>[2x]GGGAEALELLEHCGVCRERLRPEREPRLLPCLHSACSACLGPAAPAAANSSGDGGAAGDGTVVDCPVCKQQCFSKDIVENYFMRDSGSKAATDAQDANQCCTSCEDNAPATSYCVECSEPLCETCVEAHQRVKYTKDHTVRSTGPAKSRDGERTVYCNVHKHEPLVLFCESCDTLTCRDCQLNAHKDHQYQFLEDAVRNQRKLLASLVKRLGDKHATLQKSTKEVRSSIRQVSDVQKRVQVDVKMAILQIMKELNKRGRVLVNDAQKVTEGQQERLERQHWTMTKIQKHQEHILRFASWALESDNNTALLLSKKLIYFQLHRALKMIVDPVEPHGEMKFQWDLNAWTKSAEAFGKIVAERPGTNSTGPAPMAPPRAPGPLSK;>[2x]SSDSEDVVSPNCSNTVQEKTFNKDTVIIVSEPSEDEESQGLPTMARRNDDISELEDLSELEDLKD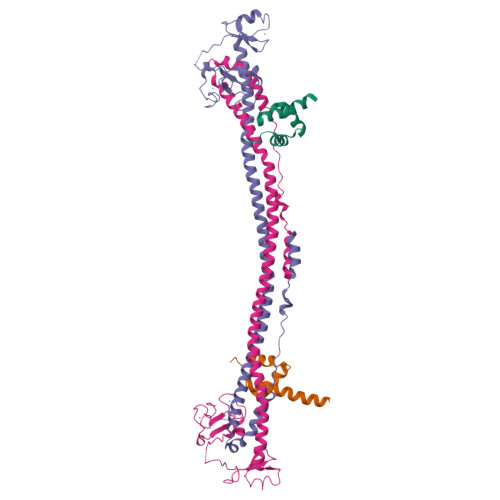AKLQTLKELFPQRSDNDLLKLIESTSTMDGAIAAALLMFGDAGGGPRKRKLSSSSEPYEEDEFNDDQSIKKTRLDHGEESNESAESSSNWEKQESIVLKLQKEFPNFDKQELREVLKEHEWMYTEALESLKVFAEDQDMQYVSQSEVPNGKEVSSRSQNYPKNATKTKLKQKFSMKAQNGFNKKRKKN> GEKTYVKRLVKILLLGAGESGKSTFLKQMRIIHGQDFDQRAREEFRPTIYSNVIKGMRVLVDAREKLHIPWGDNKNQLHGDKLMAFDTRAPMAAQGMVETRVFLQYLPAIRALWEDSGIQNAYDRRREFQLGESVKYFLDNLDKLGVPDYIPSQQDILLARRPTKGIHEYDFEIKNVPFKMVDVGGLRSERKRWFECFDSVTSILFLVSSSEFDQVLMEDRQTNRLTESLNIFETIVNNRVFSNVSIILFLNKTDLLEEKVQVVSIKDYFLEFEGDPHCLRDVQKFLVECFRGKRRDQQQRPLYHHFTTAINTENIRLVFRDVKDTILHDNLKQLMLQ;> GLIIGPEEDYDPGYFNNESDIIFQDLEKLKSHPAYLVVFLRYILSQADPGPLLFYLCSEVYQQTNP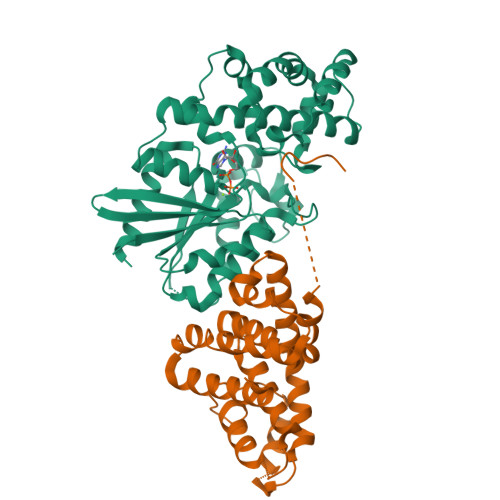KDSRSLGKDIWNIFLEKNAPLRVKIPEMLQAEIDLRLRNNEDPRNVLCEAQEAVMLEIQEQINDYRSKRTLGLGSLYGENDLLGLDGDPLRERQMAEKQLAALGDILSKYEEDRSAPMDFAVNTFMSHAGIRLRESR> MKDVVEIAVPENLVGAILGKGGK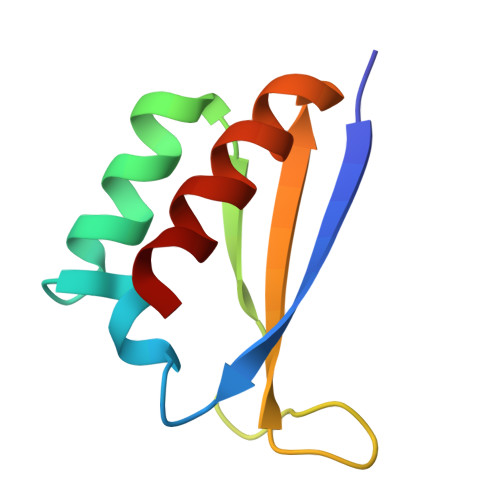TLVEYQELTGCRIQISKKGEFLPGTRNRKVTITGTPAATQAAQYLITQRI>[10x]GPLGSMTIIESNYISVREEYPDIDSE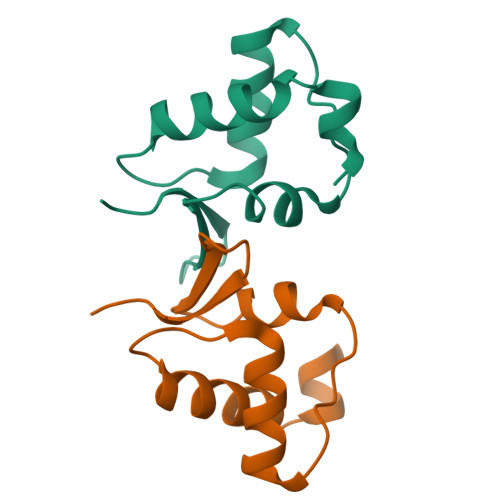VRAILLSHAQNGITISSIKSEYRKLTGNPFPLHDNVTDFLLTIPNVTAECSESGKRIFNLKAS>TPNKEDYLKCLYELGTRHNKITNKEIAQLMQVSPPAVTEMMKKLLA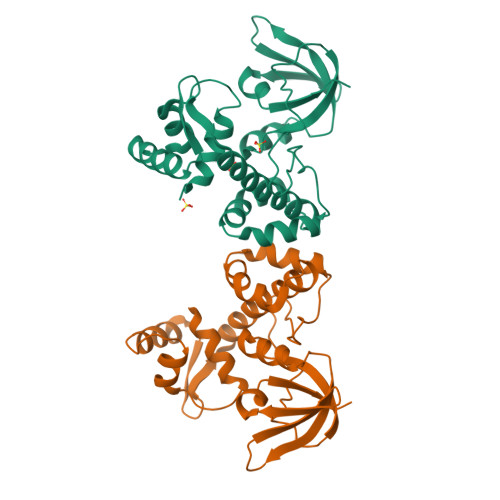EELLIKDKKAGYLLTDLGLKLVSDLYRKHRLIEVFLVHHLGYTTEEIHEEAEVLEHTVSDHFVERLDQLLDYPKACPHGGTIPAKGELLVEKHKLTLEEAKEKGDYILARVHDNFDLLTYLERNGLQVGKTIRFLGYDDFSHLYSLEVDGQEIQLAQPIAQQIYVEKI[2x]> MSENQEQ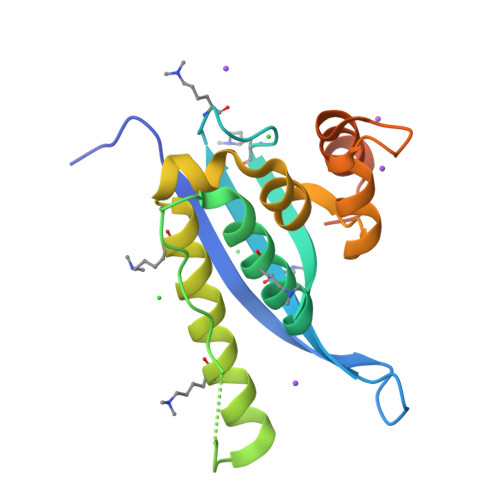EEVITVRVQDPRVQNEGSWNSYVDYKIFLHTNSKAFTAKTSCVRRRYREFVWLRKQLQRNAGLVPVPELPGKSTFFGTSDEFIEKRRQGLQHFLEKVLQSVVLLSDSQLHLFLQSQLSVPEIEACVQGRSTMTVSDAILRYAMSNCGWAQEERQSSSLEHHHHHH>SNALVRRKSATDIGGLPGKLADCRSTDPRKSELYVVEGDSAGGSAKSGRDSMFQAILPLRGKIINVEKARIDRVLKNTEVQAIITALGTGIHDEFDIGKLRYHKIVLMADADVDGQHISTLLLTLLFRFMRPLIENGHVFLAQPPLYKLKWQRSDPEFAYSDRER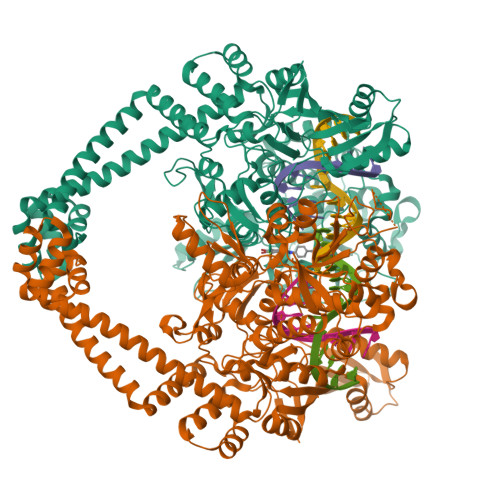DGLLEAGLKAGKKINKEDGIQRYKGLGEMDAKELWETTMDPSVRVLRQVTLDDAAAADELFSILMGEDVDARRSFITRNAKDVRFLDVTDTTLPPDDSLDRIEPVDIEQEMQRSYIDYAMSVIVGRALPEVRDGLKPVHRRVLYAMFDSGFRPDRSHAKSARSVAETMGNYHPHGDASIYDSLVRMAQPWSLRYPLVDGQGNFGSPGNDPPAAMRYTEARLTPLAMEMLREIDEETVDFIPNYDGRVQEPTVLPSRFPNLLANGSGGIAVGMATNIPPHNLRELADAVFWALENHDADEEETLAAVMGRVKGPDFPTAGLIVGSQGTADAYKTGRGSIRMRGVVEVEEDSRGRTSLVITELPYQVNHDNFITSIAEQVRDGKLAGISNIEDQSSDRVGLRIVIEIKRDAVAKVVINNLYKHTQLQTSFGANMLAIVDGVPRTLRLDQLIRYYVDHQLDVIVRRTTYRLRKANERAHILRGLVKALDALDEVIALIRASETVDIARAGLIELLDIDEIQAQAILDMQLRRLAALERQRIIDDLAKIEAEIADLEDILAKPERQRGIVRDELAEIVDRHGDDRRTRIIAIGSG[2x]> SGLVPRGSHMMEILRGSPALSAFRINKLLARFQAANLQVHNIYAEYVHFADLNAPLNDSEQAQLTRLLQYGPALSSHTPAGKLLLVTPRPGTISPWSSKATDIAHNCGLQQVDRLERGVAYYIEASTLTAEQWRQVAAELHDRMMETVFSSLTDAEKLFIHHQPAPVSSVDLLGEGRQALIDANLRLGLALAEDEIDYLQEAFTKLGRNPNDIELYMFAQANSEHCRHKIFNADWIIDGKPQPKSLFKMIKNTFETTPDYVLSAYKDNAAVMEGSAVGRYFADHNTGR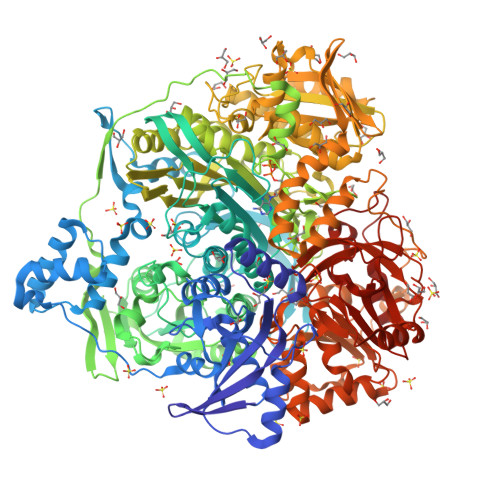YDFHQEPAHILMKVETHNHPTAISPWPGAATGSGGEIRDEGATGRGAKPKAGLVGFSVSNLRIPGFEQPWEEDFGKPERIVTALDIMTEGPLGGAAFNNEFGRPALTGYFRTYEEKVNSHNGEELRGYHKPIMLAGGIGNIRADHVQKGEIVVGAKLIVLGGPAMNIGLGGGAASSMASGQSDADLDFASVQRDNPEMERRCQEVIDRCWQLGDANPILFIHDVGAGGLSNAMPELVSDGGRGGKFELRDILSDEPGMSPLEIWCNESQERYVLAVAADQLPLFDELCKRERAPYAVIGDATEEQHLSLHDNHFDNQPIDLPLDVLLGKTPKMTRDVQTLKAKGDALNRADITIADAVKRVLHLPTVAEKTFLVTIGDRTVTGMVARDQMVGPWQVPVADCAVTTASLDSYYGEAMSIGERAPVALLDFAASARLAVGEALTNIAATQIGDIKRIKLSANWMAAAGHPGEDAGLYDAVKAVGEELCPQLGLTIPVGKDSMSMKTRWQEGNEQREMTSPLSLVISAFARVEDVRHTLTPQLSTEDNALLLIDLGKGHNALGATALAQVYRQLGDKPADVRDVAQLKGFYDAMQALVAARKLLAWHDRSDGGLLVTLAEMAFAGHCGVQVDIAALGDDHLAALFNEELGGVIQVRAEDRDAVEALLAQYGLADCVHYLGQALAGDRFVITANDQTVFSESRTTLRVWWAETTWQMQRLRDNPQCADQEHEAKANDTDPGLNVKLSFDINEDIAAPYIATGARPKVAVLREQGVASHVEMAAAFHRAGFDAIDVHMSDLLGGRIGLGNFHALVACGGFSYGDVLGAGEGWAKSILFNHRVRDEFETFFHRPQTLALGVCNGCQMMSNLRELIPGSELWPRFVRNHSDRFEARFSLVEVTQSPSLLLQGMVGSQMPIAVSHGEGRVEVRDDAHLAALESKGLVALRYVDNFGKVTETYPANPNGSPNGITAVTTENGRVTIMMPHPERVFRTVANSWHPENWGEDSPWMRIFRNARKQLG> MGSDKIHHHHHHMRTLNKDEHNYIKQIANIHETLLSQVESNYKCTKLSIALRYEMICSRLEH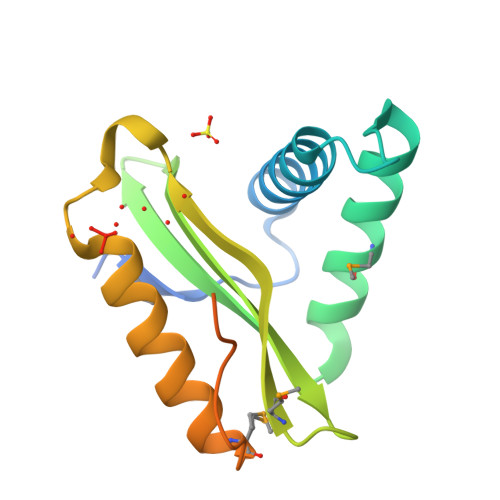TNDKIYIYENEGQLIAFIWGHFSNEKSMVNIELLYVEPQFRKLGIATQLKIALEKWAKTMNAKRISNTIHKNNLPMISLNKDLGYQVSHVKMYKDID>[2x]MSGGDGRGHNTGAHSTSGNINGGPTGLGVGGGASDGSGWSSENNPWGGGSGSGIHWGGGSGHGNGGGNGNSGGGSGTGGNLSAVAAPVAFGFPALSTPGAGGLAVSISAGALSAAIADIMAALKGPFKFGLWGVALYGVLPSQIAKDDPNMMSKIVTSLPADDITESPVSSLPLDKATVNVNVRVVDDVKDERQNISVVSGVPMSVPVVDAKPTERPGVFTASIPGAPVLNISVNNSTPAVQTLSPGVTNNTDKDVRPAFGTQGGNTRDAVIRFPKDSGHNAVYVSVSDVLSPDQVKQRQDEENRRQQEWDATHPVEAAERNYERARAELNQANEDVARNQERQAKAVQVYNSRKSELDAANKTLADAIAEIKQFNRFAHDPMAGGHRMWQMAGLKAQRAQTDVNNKQAAFDAAAKEKSDADAALSSAMESRKKKEDKKRSAENNLNDEKNKPRKGFKDYGHDYHPAPKTENIKGLGDLKPGIPKTPKQ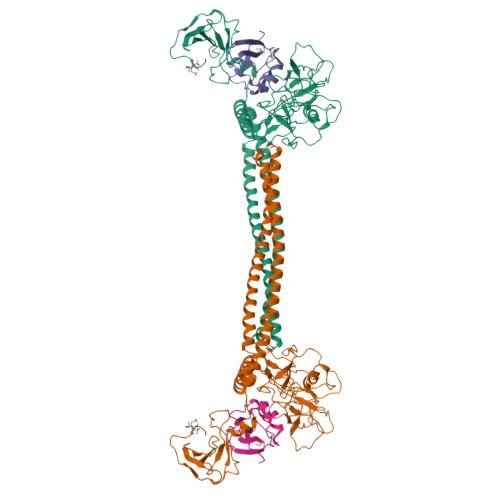NGGGKRKRWTGDKGRKIYEWDSQHGELEGYRASDGQHLGSFDPKTGNQLKGPDPKRNIKKYL;>[2x]GLKLDLTWFDKSTEDFKGEEYSKDFGDDGSVMESLGVPFKDNVNNGCFDVIAEWVPLLQPYFNHQIDISDNEYFVSFDYRDGDW> MAASKKAVLGPLVGAVDQGTSSTRFLVFNSKTAELLSHHQVEIEQKFPKEGWVEQDPKEILQSVYECIEKTCEKLGQLNIDISNIKAIGVSNQRETTVVWDKLTGEPLYNAVVWLDLRTQSTVANLSKIIPVNNNFVKTKTGLPLSTYFSAVKLRWLLDNVRKIQKAVEEDRALFGTIDSWLIWSLTGGARGGVHCTDVTNASRTMLFNIHSLEWDKELCEFFEVPMKILPNVRSSSEIYGLMKAGALEGVPISGCLGDQSAALVGQMCFQDGQAKNTYGTGCFLLCNTGHKCSVAIAGAVVRWLRDNLGIIKTSEEIEKLAKEVGTSYGCYFVPAFSGLYAPYWEPSARGIICGLTQFTNKCHIAFAALEA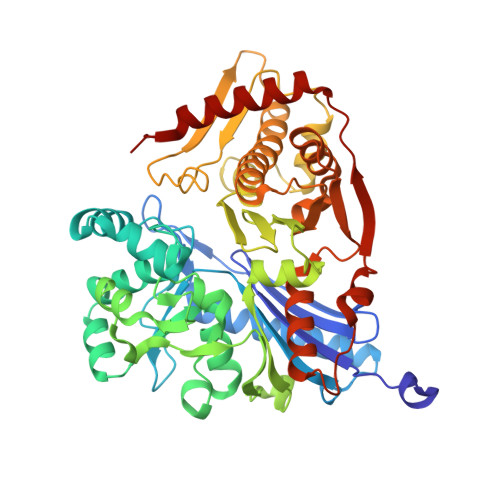VCFQTREILDAMNRDCGIPLSHLQVDGGMTNNKILMQLQADILYIPVVKPSMPETTALGAAMAAGAAEGVGVWSLKPEDLSAVTMERFEPQINAKESEIRYSTWKKAVKKSMGWV>MEDKQERANYEKLQQKFQMLMSKHQAHVRPQFESLEKINKDIVGWIKLSGTSLNYPVLQGKTNHDYLNLDFEREHRRKGSIFMDFRNELKNLNHNTILYGHHVGDNTMFDVLEDYLKQSFYEKHKIIEFDNKYGKYQLQVFSAYKTTTKDNYIRTDFENDQDYQQFLDETKRKSVINSDVNVTVKDKIMTLSTC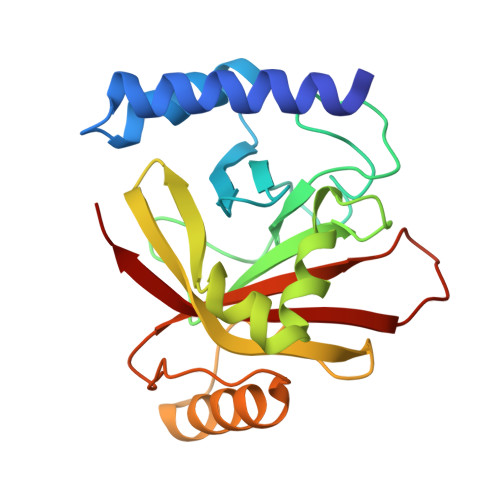EDAYSETTKRIVVVAKIIKVS[2x]>[2x]SDHKFLTQAVEEAYKGVDCGDGGPFGAVIVHNNEVVASCHN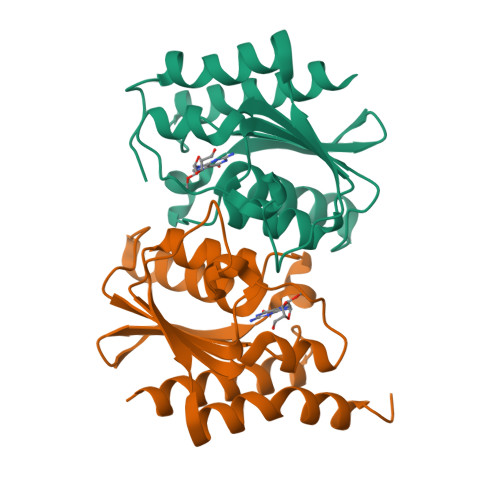MVLKYTDPTAHAQVTAIREACKKLNKIELSECEIYASCEPCPMCFGAIHLSRLKRLVYGAKAEAAIAIGFDDFIADALRGTGVYQKSSLEIKKADGNGAAIAEQVFQNTKEKFRLY>[7x]MGSSHHHHHHSSGRENLYFQGHMDIKDMKKDVKLFFFKKRIIYLTDEINKKTADELISQ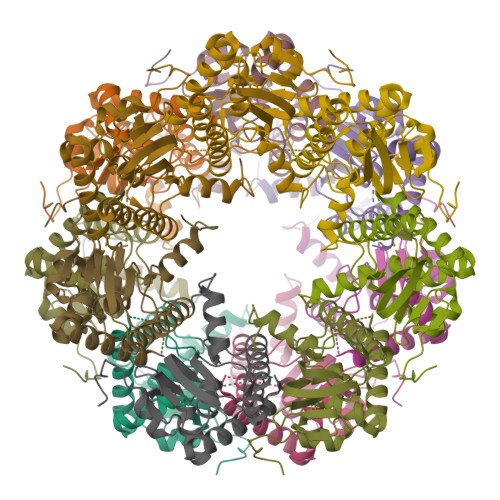LLYLDNINHNDIKIYINSPGGSINEGLAILDIFNYIKSDIQTISFGLVASMASVILASGKKGKRKSLPNCRIMIHQPLGNAFGHPQDIEIQTKEILYLKKLLYHYLSSFTNQTVETIEKDSDRDYYMNALEAKQYGIIDEVIETKLPHPYFNKVEK> CDIHVLWEWKCFE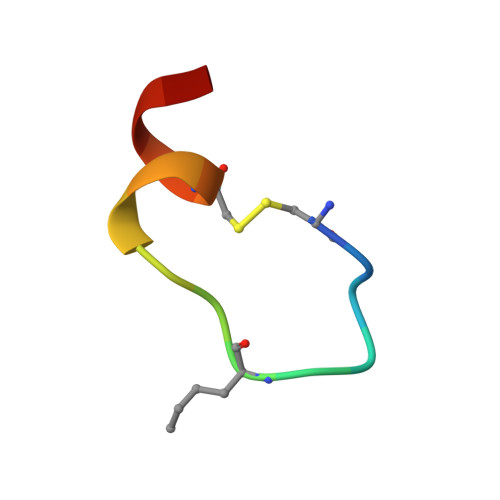DL>MGHHHHHHGEGVQLTAAQELMIQQLVAAQLQCNKRSFSDQPKVTPWPLGADPASGSASQQRFAHFTELAIISVQEIVDFAKQVPGFLQLGREDQIALLKASTIEIMLLETARRYNHETECITFLKDFTYSKDD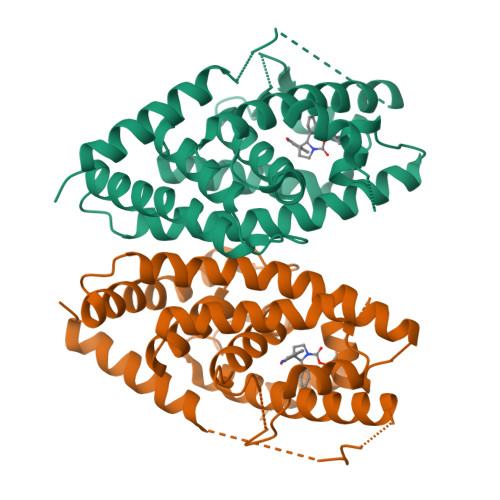FHRAGLQVEFINPIFEFSRAMRRLGLDDAEYALLIAINIFSADRPNVQEPGRVEALQQPYVEALLSYTRIKRPQDQLRFPRMLMKLVSLRTLSSVHSEQVFALRLQDKKLPPLLSEIWDVHEGSGSGSHKILHRLLQDSSS[2x]> KFFEQ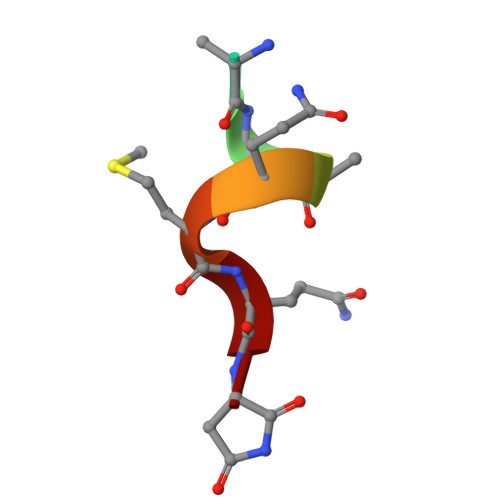MQN> GHMNVKLKVFHAGSLTEPMKAFKRAFEEKHPNVEVQTEAAGSAATIRKVTELGRKADVIATADYTLIQKMMYPEFANWTIMFAKNQIVLAYRNDSRYADEINSQNWYEILKRPDVRFGFSNPNDDPCGYRSLMAIQLAELYYNDPTIFDELVAKNSNLRFSEDNGSYVLRMPSSERIEINKSKIMIRSMEMELIHLVESGELDYFFIYKSVAKQHGFNFVELPVEIDLSSPDYAELYSKVKVVLANGKEVT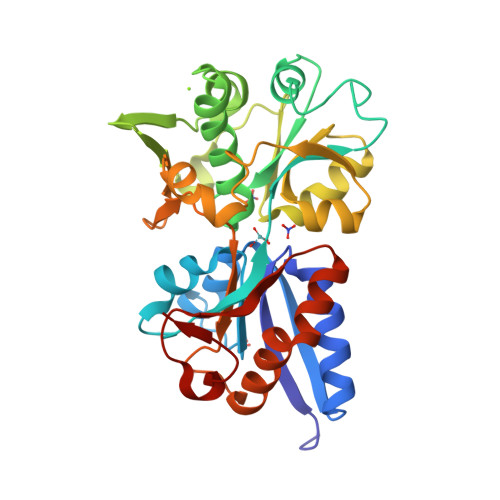GKPIVYGITIPKNAENRELAVEFVKLVISEEGQEILRELGQEPLVPPRADTAVPSLKAMVEVS> 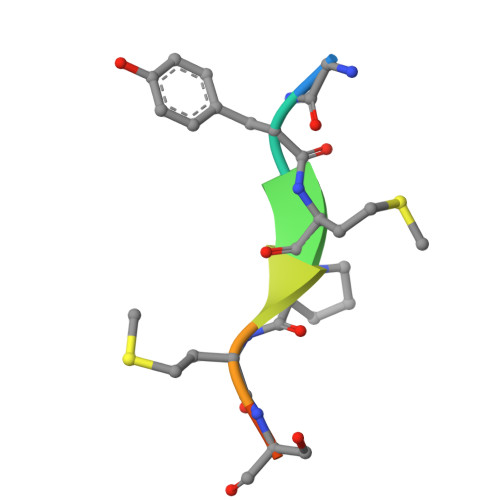GYMPMSPG>MVSVINTVDTSHEDMIHDAQMDYYGTRLATCSSDRSVKIFDVRNGGQILIADLRGHEGPVWQVAWAHPMYGNILASCSYDRKVIIWREENGTWEKSHEHAGHDSSVNSVCWAPHDYGLILACGSSDGAISLLTYTGEGQWEVKKINNAHTIGCNAVSWAPAVVPGSLIDHPSGQKPNYIKRFASGGCDNLIKLWKEEEDGQWKEEQKLEAHSDWVRDVAWAPSIGLPTSTIASCSQDGRVFIWTCDDASSNTWSPKLLHKFNDVVWHVSWSITANILAVSGGDNKVTLWKESVDGQWVCISDVNKGQGSVSASVTE[4x];>[4x]MGSSHHHHHHSGDPFSECNDEIDNAKLIMKERRFTASYTFAKFSTGSMLLTKDIVGKSGVSIKRLPTELQRKFLFDDVYLDKEIEKVTIEARKSNPYPQISESSLLFKDALDYMEKTSSDYNLWKLSSILFDPVSYPYKTDNDQVKMALLKKERHCRLTSWIVSQIGPEIEEKIRNSSNEIEQIFLYLLLNDVVRASKLAIESKNGHLSVLISYLGSNDPRIRDLAELQLQKWSTGGCSIDKNISKIYKLLSGSPFEGL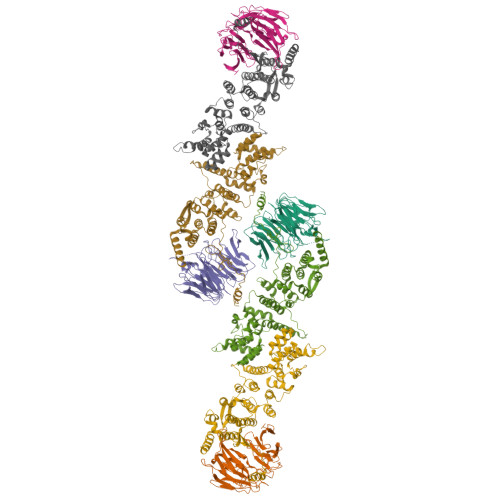FSLKELESEFSWLCLLNLTLCYGQIDEYSLESLVQSHLDKFSLPYDDPIGVIFQLYAANENTEKLYKEVRQRTNALDVQFCWYLIQTLRFNGTRVFSKETSDEATFAFAAQLEFAQLHGHSLFVSCFLNDDKAAEDTIKRLVMREITLLRASTNDHILNRLKIPSQLIFNAQALKDRYEGNYL>MGSHHHHHHDITSLYKKAGSAAAVLEENLYFGGSFTMDMAADIASDHFISRRVDIGRITLNVREKGSGPLMLFFHGITSNSAVFEPLMIRLSDRFTTIAVDQRGHGLSDKPETGYEANDYADDIAGLIRTLARGHAILVGHSLGARNSVTAAAKYPDLVRSVVAIDFTPYIETEALDALEARVNAGSQLFEDIKAV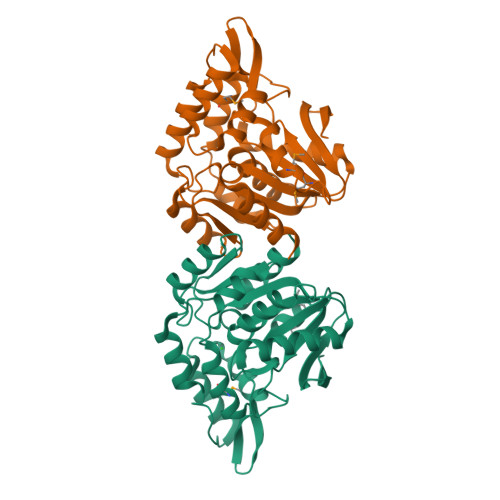EAYLAGRYPNIPADAIRIRAESGYQPVDGGLRPLASSAAMAQTARGLRSDLVPAYRDVTKPVLIVRGESSKLVSAAALAKTSRLRPDLPVVVVPGADHYVNEVSPEITLKAITNFIDA[12x]>[2x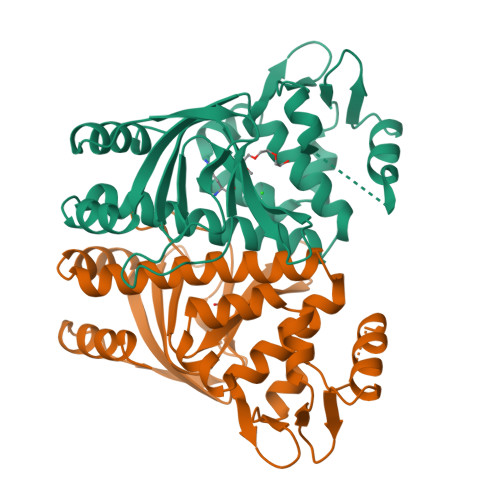]NAQAEEFKKYLETNGIKPKQFHKKELIFNQWDPQEYCIFLYDGITKLTSISENGTIMNLQYYKGAFVIMSGFIDTETSVGYYNLEVISEQATAYVIKINELKELLSKNLTHFFYVFQTLQKQVSYSLAKFNDFSINGKLGSICGQLLILTYVYGKETPDGIKITLDNLTMQELGYSSGIAHSSAVSRIISKLKQEKVIVYKNSCFYVQNLDYLKRYAPKLDEWFYLACPATWGKLN4'-bromo-N-[(2S,3R)-3-hydroxy-1-(hydroxyamino)-1-oxobutan-2-yl]biphenyl-4-carboxamide | C17 H17 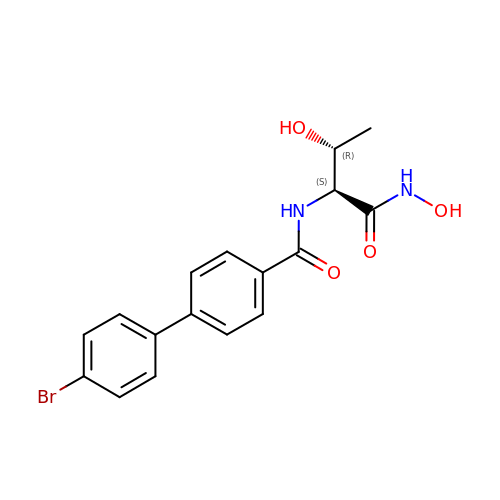Br N2 O4 | OEJYZUMESQZYFQ-BMIGLBTASA-N>MEVDPRLYFENRSKFIQDQKDKGINPYPHKFERTISIPEFIEKYKDLGNGEHLEDTILNITGRIMRVSASGQKLRFFDLVGDGEKIQVLANYSFHNHEKGNFAECYDKIRRGDIVGIVGFP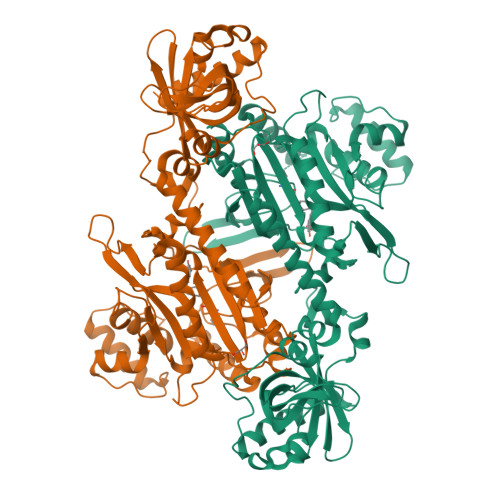GKSKKGELSIFPKETILLSACLHMLPMKYGLKDTEIRYRQRYLDLLINESSRHTFVTRTKIINFLRNFLNERGFFEVETPMMNLIAGGANARPFITHHNDLDLDLYLRIATELPLKMLIVGGIDKVYEIGKVFRNEGIDNTHNPEFTSCEFYWAYADYNDLIKWSEDFFSQLVYHLFGTYKISYNKDGPENQPIEIDFTPPYPKVSIVEEIEKVTNTILEQPFDSNETIEKMINIIKEHKIELPNPPTAAKLLDQLASHFIENKYNDKPFFIVEHPQIMSPLAKYHRTKPGLTERLEMFICGKEVLNAYTELNDPFKQKECFKLQQKDREKGDTEAAQLDSAFCTSLEYGLPPTGGLGLGIDRITMFLTNKNSIKDVILFPTMRPANGGHHHHHH[4x]> SEISRQEFQRRRQALVEQMQPGSAALIFAAPEVTRSADSEYPYRQNSD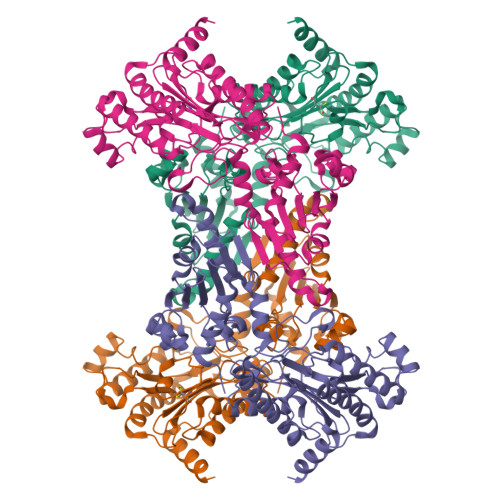FWYFTGFNEPEAVLVLIKSDDTHNHSVLFNRVRDLTAEIWFGRRLGQDAAPEKLGVDRALAFSEINQQLYQLLNGLDVVYHAQGEYAYADVIVNSALEKLRKGSRQNLTAPATMIDWRPVVHEMRLFKSPEEIAVLRRAGEITAMAHTRAMEKCRPGMFEYHLEGEIHHEFNRHGARYPSYNTIVGSGENGCILHYTENECEMRDGDLVLIDAGCEYKGYAGDITRTFPVNGKFTQAQREIYDIVLESLETSLRLYRPGTSILEVTGEVVRIMVSGLVKLGILKGDVDELIAQNAHRPFFMHGLSAWLGLDVHDVGVYGQDRSRILEPGMVLTVEPGLYIAPDAEVPEQYRGIGIRIEDDIVITETGNENLTASVVKKPEEIEALMVAARKQ>[2x]MSTQYETQGYTINNAGRRLVVDPITRIEGHMRCEVNINDQNVITNAVSCGTMFRGLEIILQGRDPRDAWAFVERICGVCTGVHALASVYAIEDAIGIKVPDNANIIRNIMLATLWCHDHLVHFYQLAGMDWIDVLDALKADPRKTSELAQSLSSWPKSSPGYFFDVQNRLKKFVEGGQLGIFRNGYWGHPQYKLPPEANLMGFAHYLEALDFQREIVKIHAVFGGKNPHPNWIVGGMPCAINIDESGAVGAVNMERLNLVQSIITRTADFINNVMIPDALAIGQFNKPWSEIGTGLSDKCVLS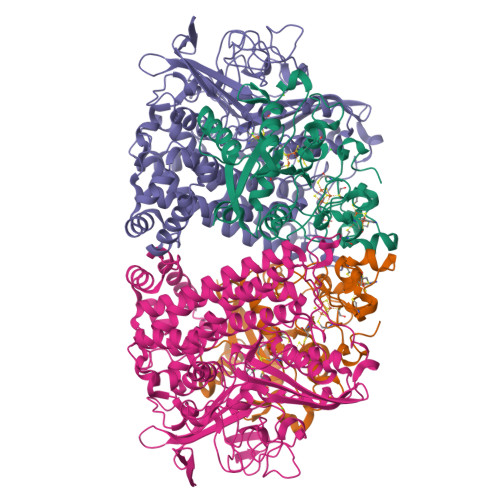YGAFPDIANDFGEKSLLMPGGAVINGDFNNVLPVDLVDPQQVQEFVDHAWYRYPNDQVGRHPFDGITDPWYNPGDVKGSDTNIQQLNEQERYSWIKAPRWRGNAMEVGPLARTLIAYHKGDAATVESVDRMMSALNLPLSGIQSTLGRILCRAHEAQWAAGKLQYFFDKLMTNLKNGNLATASTEKWEPATWPTECRGVGFTEAPRGALGHWAAIRDGKIDLYQCVVPTTWNASPRDPKGQIGAYEAALMNTKMAIPEQPLEILRTLHSFDPCLACSTH;>LENKPRIPVVWIHGLECTCCTESFIRSAHPLAKDVILSLISLDYDDTLMAAAGTQAEEVFEDIITQYNGKYILAVEGNPPLGEQGMFCISSGRPFIEKLKRAAAGASAIIAWGTCASWGCVQAARPNPTQATPIDKVITDKPIIKVPGCPPIPDVMSAIITYMVTFDRLPDVDRMGRPLMFYGQRIHDKCYRRAHFDAGEFVQSWDDDAARKGYCLYKMGCKGPTTYNACSSTRWNDGVSFPIQSGHGCLGCAENGFWDRGSFYSRVVDIPQMGTHSTADTVGLTALGVVAAAVGVHAVASAVDQRRRHNQQPTETEHQPGNEDKQARSHHHHHH[2x]>MKRYVVGISGASGIVLAVTLVSELARLGHHIDVIISPSAQKTLYYELDTKSFLSTIPQNFHNQIVLHHISSIESSVSSGSNTIDATIIVPCSVATVAAISCGLADNLLRRV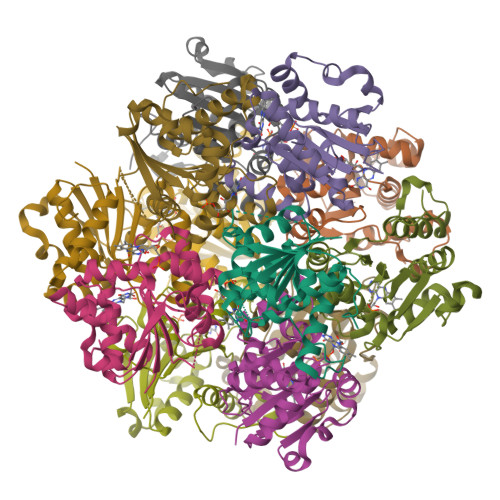ADVALKEKRPLILVPREAPLSAIHLENLLKLAQNGAVILPPMPIWYFKPQTAEDIANDIVGKILAILQLDSPLIKRWENPRLEHHHHHH[12x]> SNALAFSDMNTGAGKIENGKKALKIVVVGDGAVGKTCLLLAFSKGEIPTAYVPTVFENFSHVMKYKNEEFILHLWDTAGQEEYDRLRPLSYADSDVVLLCFAVNNRTSFDNISTKWEPEIKHYIDTAKTVLVGLKVDLRKDGSDDVTKQEGDDLCQKLGCVAYIEASSVAKIGLNEVFEKSVDCIFSN;> SNAMPPEEVVQQKFAIVAKEMKIDNPELITIPNQWKLVQEYEKKQKKDIRIQLNAQKTGNWRNAITDPKYLADLLKTRDDMDLLNEMVVVFRSSSVSFIKTFVSVGGLANLMAIYKKKIEAENSNTAIDEERKCCEVLRYVFAEEDATVALIEIDGGVELLLKGMNSKRITPDNQLDILLEITLTSSMVEHPSQEGLYLGGDVCVMNAFSNLVSEGVDMKKFLSFFSLFSKSKSEKFKHASLVLINNLIDQPELEHRMDVRNSFIEIGLVNELENMKNTEWMKIDKI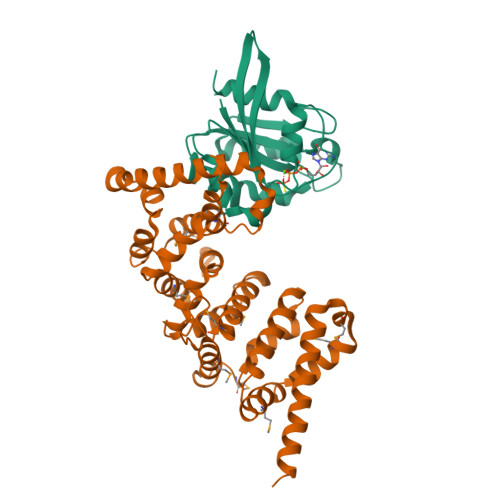KDSINDFFDSWEEDKKEVESRFDDLKQVVDFESTKSLNNYVTEQMDKFECNDILTNVHKEILFFAK>GN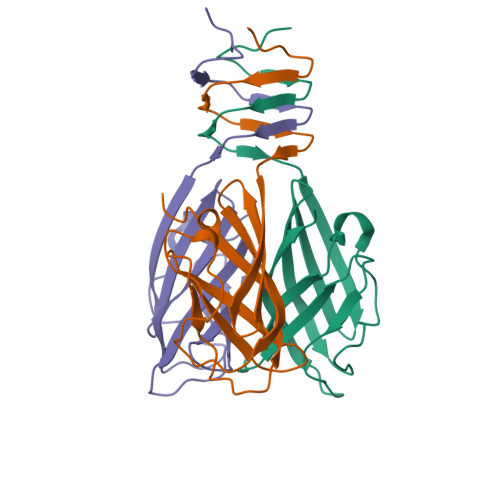VVHKTGDETIAGKKTFTGNVEVNGSLTLPVQTLTVEAGNGLQLQLTKKNNDLVIVRFFGSVSNIQKGWNMSGTWVDRPFRPAAVQSLVGHFAGRDTSFHIDINPNGSITWWGANIDKTPIATRGNGSYFIKHHH[3x]6-AMINO-3,7-DIHYDRO-IMIDAZO[4,5-G]QUINAZOLIN-8-ONE 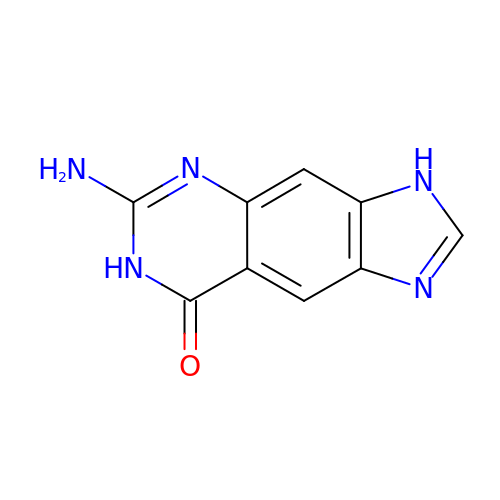| C9 H7 N5 O | VQSMWFVKBKMHTO-UHFFFAOYSA-N Glutamine synthetases (GS) catalyze the ATP-dependent ammonium assimilation, the initial step of nitrogen acquisition that must be under tight control to fit cellular needs. The dodecamer is organized as two stacked hexameric rings, and each polypeptide is organized into two parts, a shorter N-terminal domain (β-Grasp fold) and the remaining C-terminal domain. The active sites are located at the interface of the N- and C- terminal domains of the adjacent subunit in the hexameric ring. Two loops in the active center are critical for catalysis: the Glu-flap, involved in shielding the active site during catalysis and deprotonating the intermediate product, and the Asp-50’ loop, which binds and deprotonates ammonium.

The complex with 2OG/Mg2+ was obtained with and without ATP (MtGS-2OG/Mg2+/ATP, MtGS-2OG/Mg2+) in a new crystalline form and both were refined to 2.15 Å and 2.91 Å resolution, respectively. Since the 2OG/Mg2+/ATP complex is at a higher resolution, this structure was preferred for deeper structural analyses. The allosteric 2OG binding site, ~15 Å distant from the catalytic cleft, is localized at the interface between the C-terminal domain and the adjacent N-terminal domain. 2OG is coordinated via ionic bonds by Arg20´, Arg88´, Arg174, Arg175 and a hydrogen bond via Ser191 (primed numbers indicate the adjacent unit). Phe18ʹ stabilizes the 2OG via stacking with its phenyl ring. 2OG presence at the interface of monomers reorients the bulky side chain of Phe18’, and remodels salt bridge networks in its surrounding. Consequently, the N-terminal domain is pushed away from the neighboring C-terminal domain, and the α-helix 6 and β-hairpin 9-10 (residues 167-206, in the vicinity of the active site) are shifted. In the MtGS-2OG/Mg2+/ATP structure, the ATP is located in a similar position compared to bacterial homologs. Strikingly, in the 2OG-bound state of MtGS, the 318-325 and Asp50´-loops adopt a position similar to all described active transition states in bacterial homologs. This suggests that the binding of 2OG triggers conformational changes leading to a catalytically competent conformation and explaining the 2OG dependency for activity.

>[12x]MSTVEQVLEYVKSNNVKFMRFQFVDILGVPKNVAFPIKAGEKGIEELRDVLENGLYFDGSSIEGFVGINESDMMLKPDLSTFSVLPWRPSEKSVARVICDVYTTKGKPFEGDPRGCLKRVMEEFKKEFNGEYFVGPEPEFFLLKKDPHNPHKYIPADDGGYFDLEPMDEAPDIRRDIVFALENLGFHVEASHHEVAPGQHEVDFKFDDALKTADSVITFKTTIKTIAEQHGLKATFMPKPFFGMNGSGMHCHQSIWLNGEPSFYDENAPYQLSETCMNYVAGILKHAKAIVAITNPTVNSYKRLVPGYEAPVNIAWANSNRSAIIRVPAARGKGTRIEFRAPDPSCNPYLAFTVMLAAGLDGVKNKLDAPEPVERNIFAMSEAEKKELGIESVPANLKAALDELENNDVLKNALGKHIFESFLEIKNAEWDSFRTSVTDWETTAYLKI The RNA genome sizes of LSV1 and LSV2 are ~5.6 kb, encoding three major genes: the Orf1 with the unclear function, RdRP responsible for viral RNA replication, and the capsid protein (CP) for the host recognition and viral capsid assembly. CP forms the capsid shell that protects genomes and is responsible for both host specificity and receptor binding to transport the viral genome into infected host cells, or for intracellular trafficking. We determine cryo-EM structures of T = 4 and T = 3 capsids of virus-like particles (VLPs) of Lake Sinai virus (LSV) 2 and delta-N48 LSV1, belonging to tetraviruses, at resolutions of 2.3–2.6 Å in various pH environments. Analyses of these capsid structures reveal the intermolecular interactions that drive subunits assembly into homo-trimeric capsomeres and eventually into a complete viral capsid in which specific domains, such as the N-terminal domain, the helical domain, and the β-barrel domain/C-arm, could encapsidate nucleic acids.

The models of T = 4 and T = 3 LSV2 VLPs were built and refined with the homo-trimeric subunits A/B/C or D/D/D. Each icosahedral asymmetric unit (iASU) of the T = 4 particle consists of four subunits A, B, C, and D, whereas one iASU of the T = 3 particle comprises A, B, and C subunits with the C/C dimer taking up a position similar to the C/D dimer of T = 4 particles. Accordingly, the T = 4 LSV2 VLP is an icosahedral symmetrical sphere consisting of 240 copies of the 57-kDa full-length CP with 80 apparent trimeric spikes on the VLP surface, whereas the T = 3 LSV2 VLP is composed of 180 copies with 60 trimeric spikes. As a result, the T = 4 and T = 3 particle sizes of LSV2 VLP are variable, with diameters ranging from 494 to 482 Å and 450 to 438 Å, respectively, from alkaline (pH 8.5) to acidic (pH 6.5) conditions. In comparison to the expanded T = 4 and T = 3 particles at the neutral or basic pH condition, measurements of diameters of the shaped holes on the I5 and I2 axes of the unexpanded particles at pH 6.5 show that the minimum and maximum displacements were changed from ~5 to 4 Å and from ~22 to 15.5 Å, respectively. At a neutral or basic pH environment, homo-trimeric subunits A/B/C rotate along I5 axes; homo-trimeric subunits D/D/D raise around I2 axes, leading the iASU to pivot upward. In contrast, the basis of the quaternary change on the T = 4 and T = 3 particles at acidic pH is further flattened on the I2 and I3 axes, respectively, suggesting flattened hexameric capsomeres concomitantly result in a compact particle. Furthermore, the superimposition Cα of CPs between T = 4 and T = 3 LSV2 VLPs at a neutral (or basic) and acidic pH shows no obvious change.

>MNPPTTTTTTTRTIRAPKVQLTPNSATRRRRNRRRRRPAAAIAGPLSIQPSSINRRMVSRVTRRSAVVTAAGLAWLRQYLNPMGPDTTSVTGYPDGSAVTTCIADYSNTFNVSFPPREALYCTGSSSSEKPTLVDADNYAKIDKWSNYDITLCVLALPMLRNVVMLRLYPHTPTAFALTEQTPNFPQRFPNWSVYSADGTRFNNGDEPGYLQSYVYLPNVDKHLSAARGYRLLSRGITGIFSAPALETQGFVTACQYLAEGSIQSQSIKSDAVRSVTVNSDGTVKNVESSSQTVSSMPRYVFPLDGDNCAPSSLTETYHQAYQSKATDGFYMPVLSSSRDNPFHPPQPRAIAVYGSFLARGCLDPVSEAHEADGPTHDIYRLNVADDVAPLFNTGVVWFEGISPKFSLKLKTRTVLQYIPTSGSVLANFTRHEPTYDQIALDAADRLRNLMPHAYPAAYNDWGWLGDLLDSAISMLPGVGTVYNIAKPLIKPAWNWLGNKVSDFFGNPVARDGDIFFDAK[4x]> SSHHHHHHMSGENLYFQGASAAIVTDTGGVDDKSFNQSAWEGLQAW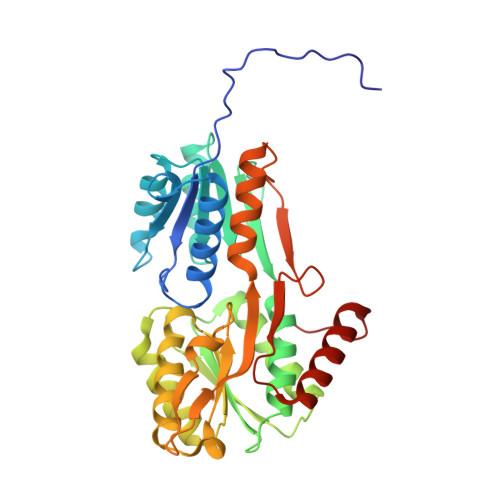GKEHNLSKDNGFTYFQSTSEADYANNLQQAAGSYNLIFGVGFALNNAVKDAAKEHTDLNYVLIDDVIKDQKNVASVTFADNESGYLAGVAAAKTTKTKQVGFVGGIESEVISRFEAGFKAGVASVDPSIKVQVDYAGSFGDAAKGKTIAAAQYAAGADIVYQVAGGTGAGVFAEAKSLNESRPENEKVWVIGVDRDQEAEGKYTSKDGKESNFVLVSTLKQVGTTVKDISNKAERGEFPGGQVIVYSLKDKGVDLAVTNLSEEGKKAVEDAKAKILDGSVKVPE>[4x]MLPKATVKRIMKQHTDFNISAEAVDELCNMLEEIIKITTEVAEQNARKEGRKTIKARDIKQCDDERLKRKIMELSERTDKMPILIKEMLNVITSEL

Archaeal histones are dimeric and assemble on DNA into ‘hypernucleosome’ particles of varying sizes with each dimer wrapping 30 bp of DNA. Here, we characterise the structure and function of the histone paralogue MJ1647 from Methanocaldococcus jannaschii that has a unique C-terminal extension enabling homotetramerisation. Unlike canonical histones, MJ1647 tetramers can bridge two DNA molecules in vitro. To the best of our knowledge, MJ1647 is the first histone shown to have DNA bridging properties, which has important implications for genome structure and gene expression in archaea.

To elucidate the role of the MJ1647 tetramerisation module in oligomerisation and DNA binding, we solved the molecular structure of the MJ1647 histone by crystallisation and X-ray diffraction at 1.9 Å resolution. MJ1647 crystallised as dimers and the refined model shows that each monomer contains the classic histone fold (three α-helices separated by two loops) with a very strong correspondence to well-characterised archaeal histones such as HMfB, including the electrostatic surface charge distribution. Unlike the disordered tails of eukaryotic histones, the MJ1647 tetramerisation module forms a well-structured region of the protein and is composed of two α-helices separated by a loop. The two helices from each monomer are packed against each other to create an interleaved or ‘hand-shake’ arrangement, adding considerably to the overall interaction surface between monomers in the dimer. The dimers in the crystal structure differ to the tetrameric state of the protein in solution observed in SEC-MALS and native mass spectrometry experiments. This discrepancy is possibly due to the low pH (4.6) in the crystallisation buffer that could favour MJ1647 dimers. Unable to obtain crystals of the MJ1647 tetramer at higher pH, we generated structural models for MJ1647 tetramers using the structure prediction algorithm AlphaFold2. While TM helices 4 and 5 form monomer–monomer interactions within MJ1647 dimers in the crystal structure, TM helices 4 and 5 ‘open up’ in the tetrameric model and make new interactions with opposing monomers that enable dimer–dimer interactions within the tetramer. By comparison, the distance between positions 80 and 95 of monomers within the dimer of the crystal structure (11.1 Å) is incompatible with disulfide bond formation. Overall, our crystallisation results suggest that MJ1647 might exist in an alternative state next to the dominant tetrameric state we observed in our biochemical assays.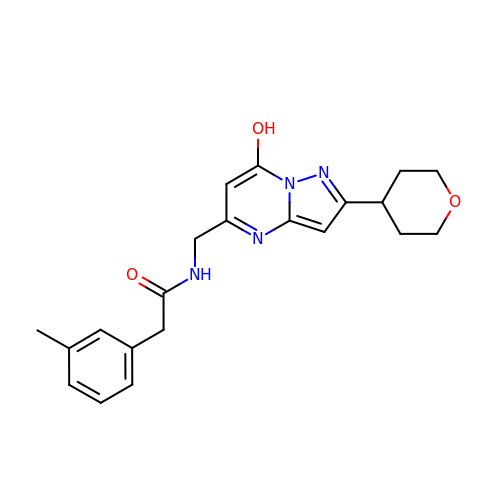2-(3-methylphenyl)-~{N}-[[2-(oxan-4-yl)-7-oxidanyl-pyrazolo[1,5-a]pyrimidin-5-yl]methyl]ethanamide | C21 H24 N4 O3 | WQHBERINDYVLKU-UHFFFAOYSA-N> MEGSIKEIAITHHVKEGHEKADPSQFELLKVLGQGSFGKVFLVKKISGSDARQLYAMKVLKKATLKVRDRVRTKMERDILVEVNHPFIVKLHYAFQTEGKLYLILDFLRGGDLFTRLSKEVMFTEEDVKFYLAELALALDHLHSLGIIYRDLKPENILLDEEGHIKLTDFGLSKESIDHEKKAYSFCGTVEYMAPEVVNRRGHTQSADWWSFGVLMFEMLTGTLPFQGKDRKETMTMILKAKLGMPQFLSPEAQSLLRMLFKRNPANRLGAGPDGVEEIKRHSFFSTIDWNKLYRREIHPPFKPATGRPEDTFYFDPEFTAKTPK

The 90-kDa ribosomal S6 kinase 2 (RSK2) is a serine-threonine kinase, which plays a key role in the mitogen-activated protein (MAP) kinase signaling pathway. Among the many serine-threonine kinases, only two unique kinases, RSK and MSK, contain two distinct kinase domains in a single polypeptide chain, separated by a linker region of ∼100 amino acids. Both domains are catalytically functional, and the C-terminal kinase domain (CTD) regulates the activity of the N-terminal domain (NTD) through phosphorylation of the hydrophobic linker region. The activated CTD RSK2 autophosphorylates Ser386 in the linker region, which becomes a docking site for PDK1 that activates the NTD RSK2 through phosphorylation of Ser227 in the T-activation loop.

The X-ray crystal structure of the N-terminal kinase domain of RSK2 (residues 44–367) complexed with AMP-PNP was refined to 1.8 Å resolution. The NTD RSK2 adopted an overall protein kinase two-lobal scaffold with the ATP-binding site in the cleft between the small N-terminal lobe and large α-helical C-terminal lobe. The T-activation loop (residues 220–230), part of the αC-helix (residues 111–119), and the N- and C-termini (residues 44–46 and 347–367, respectively) were not visible in the electron density map and were not included in the current model. The βB-sheet insert is comprised of three antiparallel β-strands: the β-1-strand (residues 48–52) at the N-terminal end; the novel βB-strand (residues 104–109); and the β9-strand of the activation segment (residues 215–217). In the NTD RSK2 structure, the αC-helix is pushed away from its regular position by the βB-sheet, and consequently, the conserved Glu118 residue (invisible in the structure) from the αC-helix cannot interact with Lys100. The lysine, located on the βB-sheet, interacts with the β-phosphate (distance 2.66 Å) and the conserved Asp211 (distance 2.86 Å) from the DFG-motif. Instead of the salt bridge, Lys100-Glu118, a new mode of connection appeared – Lys100-β-phosphate-Lys216. Surprisingly, the isolated NTD RSK2 displayed in vitro kinase activity toward the S6 peptide even without activation by PDK1. We present a kinase structure that would be classified as having an “inactive” conformation (the displaced αC-helix), but is actually an active phosphorylated kinase confirmed by complementary protein activity assay. Whereas in PKB this region is occupied by the C-terminal hydrophobic motif (HM), in the NTD RSK2, the N-terminal β0-strand (residues 55–57) is anchored to that groove by several hydrogen bonds with the β4-strand.> MAPKKQEQEPIRLSTRTASKKVDYLQLSNGKLEDFFD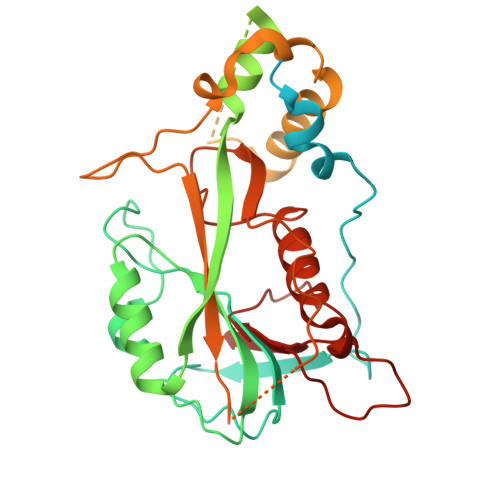DLEEDNKPARNRSRSKKRGRKPLKKADSRSKTPSRVSNARGRSKSLGPRKTYPRKKNLSPDNQLSLLLKWRNDKIPLKSASETDNKCKVVNVKNIFKSDLSKYGANLQALFINALWKVKSRKEKEGLNINDLSNLKIPLSLMKNGILFIWSEKEILGQIVEIMEQKGFTYIENFSIMFLGLNKCLQSINHKDEDSQNSTASTNNTNNEAITSDLTLKDTSKFSDQIQDNHSEDSDQARKQQTPDDITQKKNKLLKKSSVPSIQKLFEEDPVQTPSVNKPIEKSIEQVTQEKKFVMNNLDILKSTDINNLFLRNNYPYFKKTRHTLLMFRRIGDKNQKLELRHQRTSDVVFEVTDEQDPSKVDTMMKEYVYQMIETLLPKAQFIPGVDKHLKMMELFASTDNYRPGWISVIEK> MARSKIALIGAGQIGGTLAHLAGLKELGDVVLFDIVDGVPQGKALDIAESAPVDGFDAKYSGASDYSAIAGADVVIVTAGVPRK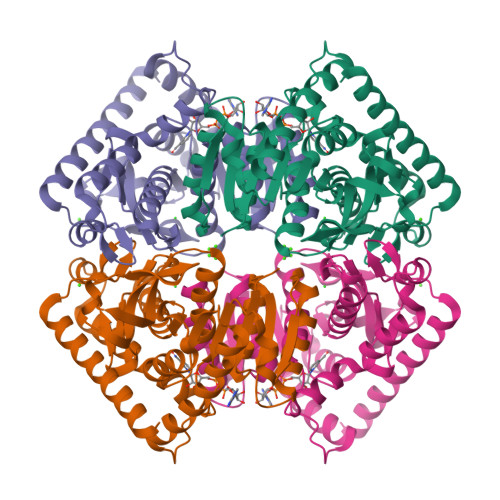PGMSRDDLIGINLKVMEAVGAGIKEHAPDAFVICITNPLDAMVWALQKFSGLPTNKVVGMAGVLDSARFRHFLAEEFGVSVEDVTAFVLGGHGDDMVPLTRYSTVAGVPLTDLVKLGWTTQEKLDAMVERTRKGGGEIVNLLKTGSAFYAPAASAIAMAESYLRDKKRVLPCAAYLDGQYGIDGLYVGVPVVIGENGVERVLEVTFNDDEKAMFEKSVNSVKGLIEACKSVNDKLA> GPQIASMSATALLQKAAQ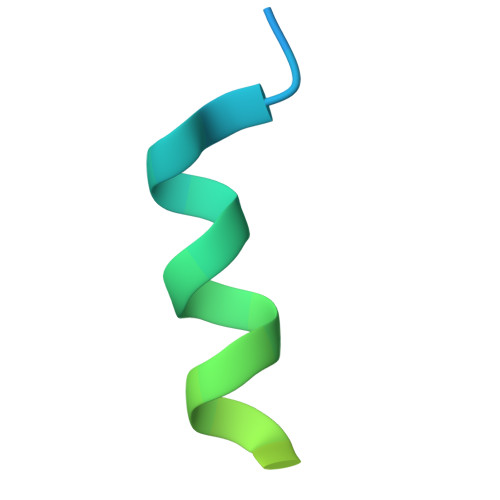MGSKRSSSSSSNSKTFGLMT>[2x]MVSGEVRTKKVPLDTNHKRFYDAFAQGAGKLDLDRQCVECHHEKPGGI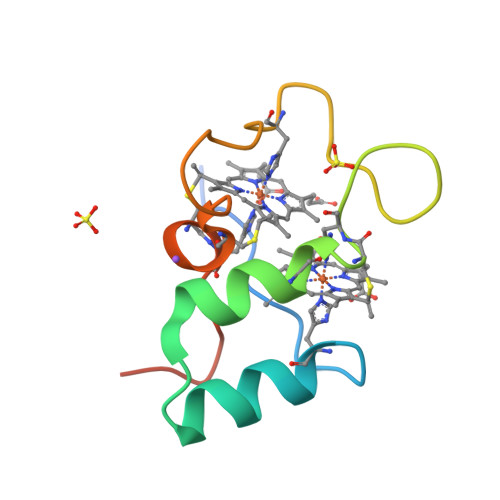PFPKNHPVKPADGPMRCLFCHKFKLEHHHHHH>[4x]GAGAGAGAGAGMEQT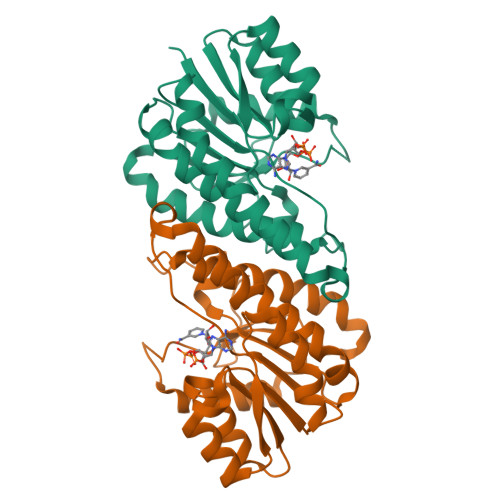YFISGANRGIGFSVVQRLAAKSGVKVIATARDPASATALNELAKENPQVKVVQLDISDEESIKKIAKNVSQYTDSIDVFVSNAAIAKSFGPLLNTPREQWIEHFFTNVLGPIRLFQELYPLIKKGTQKKVFFISSNAGSLNLDFGLDFSAYGQSKAALNYSTKELARQLKPENFIVAAVHPGVVTTDMGKGGERAFTAVDEVSAKKFFTPETKITPEESAAALCKLFESLNTTGKYLSYDGTELPW>[9x]MEDINFASLAPRHGTRPFMGTWNEIGTSQLNGGAFNWSSVWSGLKNFGSTLRTYGNKAWNSSTGQLLREKLKDQNFQQKVVDGLASGINGVVDIANQAVQREINSRLDPRPPTVVEMEDATLPPPKGEKRPRPDAEETILQVDEPPSYEEAVKAGMPTTRIIAPLATGVMKPATLDLPPPPAPAPPKATPVVQAPPVATAVRRVPARRQAQNWQSTLHSIVGLGVKSLKRRRCY;>MATPSMMPQWAYMHIAGQDASEYLSPGLVQFARATDTYFSLGNKFRNPTVAPTHDVTTDRSQRLTLRFVPVDREATTYLYKARFTLAVGDNRVLDMASTYFDIRGVLDRGPSFKPYSGTAYNSLAPKGAPNPSQWETKEKQGTTGGVQQEKDVTKTFGVAATGGINITNQGLLLGTDETAENGKKDIYADKTFQPEPQVGEENWQENEAFYGGRALKKDTKMKPCYGSFARPTNEKGGQAKFKPVNEGEQPKDLDIDFAYFDVPGGSPPAGGSGEEYKADIILYTENVNLETPDTHVVYKPGTSDNSSEINLVQQSMPNRPNYIGFRDNFVGLMYYNSTGNMGVLAGQASQLNAVVDLQDRNTELSYQLLLDSLGDRTRYFSMWNSAVDSYDPDVRIIENHGVEDELPNYCFPLNGTGTNSTYQGVKITNGNDGAEESEWEKDDAISRQNQICKGNVYAMEINLQANLWKSFLYSNVALYLPDSYKYTPANVKLPANTNTYEYMNGRVVAPSLVDAYINIGARWSLDPMDNVNPFNHPRNAGLRYRSMLLGNGRYVPFHIQVPQKFFAIKNLLLLPGSYTYEWNFRKDVNMILQSSLGNDLRVDGASVRFDSVNLYATFFPMAHNTASTLEAMLRNDTHDQSFNDYLSAANMLYPIPAKATNVPISIPSRNWAAFRGWSFTRLKTKETPSLGSGFDPYFVYSGSIPYLDGTFYLNHTFKKVSIMFDSSVSWPGNDRLLTPNEFEIKRSVDGEGYNVAQCNMTKDWFLVQMLSHYNIGYQGFHVPEGYKDRMYSFFRNFQPMSRQVVDEINYKDYKAVTLPFQHNNSGFTGYLAPTMRQGQPYPANFPYPLIGQTAVPSVTQKKFLCDRVMWRIPFSSNFMSMGALTDLGQNMLYANSAHALDMTFEVDPMDEPTLLYLLFEVFDVVRVHQPHRGVIEAVYLRTPFSAGNATT[12x];> MSQQAPDPAIRAALQSQPSGLASDDWEAAMQRIMALTTRNPESFRQQPQANRLSAILEAVVPSRTNPTHEKVLAIVNALAENKAIRPDEAGLVYNALLERVGRYNSTNVQSNLDRLVTDVREAVAQRERFKNEGLGSLVALNAFLATQPANVPRGQDDYTNFISALRLMVTEVPQSEVYQSGPDYFFQTSRQGLQTVNLSQAFKNLRGLWGVQAPVGDRSTVSSLLTPNSRLLLLLIAPFTDSGSVNRNSYLGHLLTLYREAIGQAQVDEQTFQEITSVSRALGQNDTDSLRATLNFLLTNRQQKIPAQYALSAEEERILRYVQQSVGLFLMQEGATPSAALDMTARNMEPSMYAANRPFINKLMDYLHRAAAMNTDYFTNAILNPHWLPPPGFYTGEYDMPDPNDGFLWDDVDSAVFSPTFQKRQEAPPSEGAVGRSPFPSLGSLHSLPGSVNSGRVSRPRLLGEDEYLNDSLLQPPRAKNAMANNGIESLVDKLNRWKTYAQDHRDAPAPRRQRHDRQRGLVWDDEDSADDSSVLDLGGSGGVNPFAHLQPKLGRRMF;> MRRAVVSSSPPPSYESVMAQATLEVPFVPPRYMAPTEGRNSIRYSELAPQYDTTRVYLVDNKSADIASLNYQNDHSNFLTTVVQNNDFTPAEASTQTINFDERSRWGGDLKTILHTNMPNVNEYMFTSKFKARVMVSRKHPEGVVETDLSQDKLEYEWFEFTLPEGNFSETMTIDLMNNAILENYLQVGRQNGVLESDIGVKFDSRNFKLGWDPVTKLVMPGVYTYEAFHPDVVLLPGCGVDFTESRLSNLLGIRKKQPFQEGFRIMYEDLEGGNIPALLDVPKYLESKKKVEDETKNAAAATADTTTRGDTFATPAQETAADKKVEVLPIEKDESGRSYNLIQGTHDTLYRSWYLSYTYGDPEKGVQSWTLLTTPDVTCGAEQVYWSLPDLMQDPVTFRSTQQVSNYPVVGAELMPFRAKSFYNDLAVYSQLIRSYTSLTHVFNRFPDNQILCRPPAPTITTVSENVPALTDHGTLPLRSSIRGVQRVTVTDARRRTCPYVYKALGIVAPRVLSSRTF;> MAKRLRVEDDFNPVYPYGYARNQNIPFLTPPFVSSDGFKNFPPGVLSLKLADPITINNGDVSLKVGGGLAVEQQTGNLSVNPDAPLQVASDKLQLALAPPFEVRDGKLALKAGNGLKVLDNSITGLTGLLNTLVVLTGRGIGTEELKNDDGVTNKGVGLRVRLGDDGGLTFDKKGDLVAWNKKDDRRTLWTTPDTSPNCKMSTEKDSKLTLTLTKCGSQVLGNVSLLAVTGEYHQMTATTKKDVKISLLFDENGILLPSSSLSKDYWNYRSDDSIVSQKYNNAVPFMPNLTAYPKPSAQNAKNYSRTKIISNVYLGALTYQPVIITIAFNQETENGCAYSITFTFTWQKDYSAQQFDVTSFTFSYLTQENKDKD;>MNGTGGAFEGGLFSPYLTTRLPGWAGVRQNVMGSTVDGRPVLPANSSTMTYATVGNSSLDSTAAAAAAAAAMTATRLASSYMPSSGSSPSVPSSIIAEEKLLALLAELEALSRQLAALTQQVSELREQQQQQNK[4x];>[2x]MSKEIPTPYMWSYQPQMGLAAGASQDYSTRMNWLSAGPSMISRVNGVRSHRNQILLEQAAVTSTPRAKLNPRNWPSTLVYQEIPGPTTVLLPRDALAEVRMTNSGVQLAGGASRCPLRPQSGIKTLVIRGRGTQLNDELVSSSIGLRPDGVFQLAGAGRSSFTPNQAYLTLQSSSSEPRSGGIGTLQFVEEFVPSVYFNPFSGSPGLYPDEFIPNFDAVREAVDGYD

Human adenovirus D26 (HAdV-D26, or Ad26 for short) causes acute conjunctivitis and a prolonged enteric infection among humans. Significantly, Ad26 is being used as a vaccine vector against the diseases such as SARS-CoV-2 and AIDS. In addition to differences in the hypervariable regions (HVRs), Ad26 displays a short-shafted fiber comprising eight β-spiral repeats, compared with long-shafted fibers found in archetypal HAdV-C5. The overall structure and capsid protein organization of the HAdV-D26 capsid is very similar to that of HAdV-C5.

Here, we report the improved capsid structure for one of these vectors, human adenovirus D26 (HAdV-D26), at 3.4 Å resolution, by reprocessing the previous cryo-electron microscopy dataset and obtaining a refined model. Using this higher resolution map, we obtained a refined model for Ad26 capsid by performing real-space refinement using Phenix and model building in Coot, providing new insights into the structures and organization of minor proteins, IIIa, VI, and VIII, which were not previously considered. Not surprisingly, the significant structural differences between the hexons from Ad26 and Ad5 occur in the HVR loops. It is noteworthy that all HVRs, including HVR1, are ordered in the Ad26 hexon. Moreover, the FNT-peptide adopts “elbow” shaped conformation that appears to hook the helix at the base of the disordered RGD containing loop, which perhaps is critical for fiber latching onto PB. The Ad26 structure provided the first report of a well-ordered full-length protein-IX (IX) that revealed the connection (linker region) between the triskelion and coiled-coil forming regions in HAdVs. It appears that the APD domain in Ad26-IIIa is rotated by ~120°, compared with its counterpart in the Ad5-ts1 structure, which results in a longer distance (by ~25 Å) between the visible ends of MDLD and APD domains. It is noteworthy that this reorganization of the APD domain in the Ad26 structure results in the loss of interactions with the contacting hexon subunits. Notably, except for the ordered short segment of the processed peptide (140–149), the rest of the VIII structure is very similar in Ad26 and Ad5 virions. In the refined Ad26 structure, the directionality of the polypeptide chains of pVIn in the previous structure was reversed in agreement with the recent Ad5-wt and ts1 virion structures. Furthermore, we identified two, two, three, and two copies of pVIn bound in the hexons 1–4, respectively.> 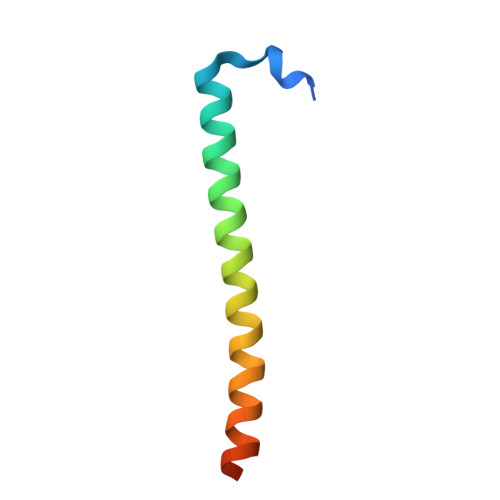GSEVEWDAFSIPELQNFLTILEKEEQDKIQQVQKKYDKFRQKLEEALRESQGKPG>[4x]MSLSGPRVERLEVSAYTVPTDYPESDGTLQWDSTTMILVEAHGGGRKGLGYTYGDVSVGRFVESKLAGVAEGSDALSPPAVWARMQAAIRNAGRPGVGAMAVSAVDIALWDLKARLLGLPLADALPRFHAEVPVYGSGGFTSYPLRRLQEQLGGWAAAGIPRVKMKVGREPEKDPERVRAAREAIGESVELMVDANGAYTRKQALYWAGA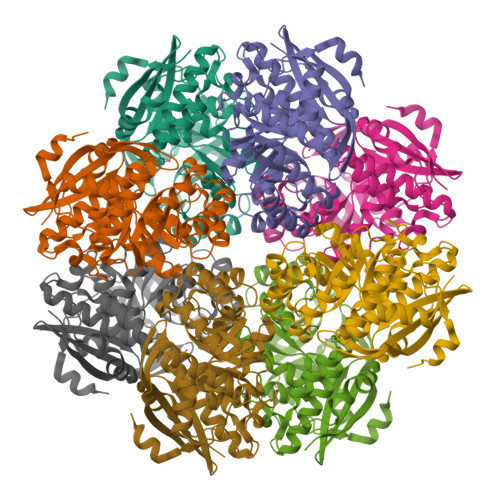FAREAGISYLEEPVSSEDREGLRLLRDRGPGGVAIAAGEYEWTLPQLHDLAGCVDILQADVTRCGGITGLLRVDGICRGHQIPFSAHCAPAVSAHACCAVESLLHLEYFHDHARVERLLFDGTLDPEGGSLRPDPDRPGLGLELKRSEAGKYAAEGHHHHHH> SALYAPSALVLTVGKGVSATTAAPERAVTLTCAPGPSGTHPAAGSACADLAAVGGDL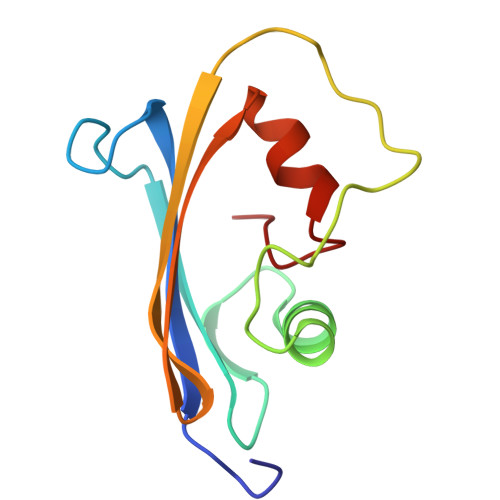NALTRGEDVGCPKVYDPVLLTVDGVWQGKRVSYERVFSNECEMNAHGSSVFAF>[2x]MAPKCIECHINIEMDPVLHDVFKLQVCKQCSKEHPEKYALLTKTECKEDYFLTDPELNDEDLFHRLEKPNPHSGTFARMQLFVRCEVEAFAFKKWGGEEGLD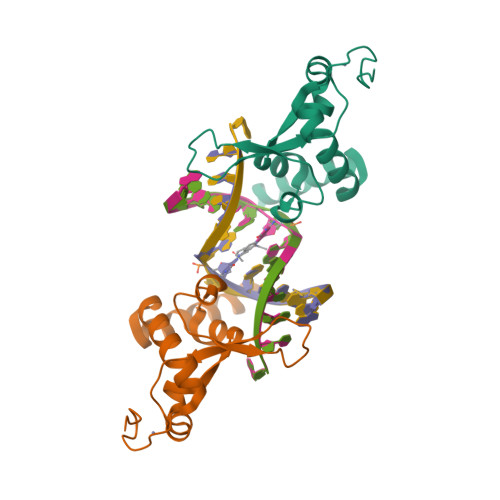EEWQRREEGKAHRREKKYGSAWSHPQFEK>AKEMQNVPYTIAVDGIMAFNQSYLNLPKDSQLSYLDLGNKVKALLYDERGVTPEKIRNAKSAVYTITWKD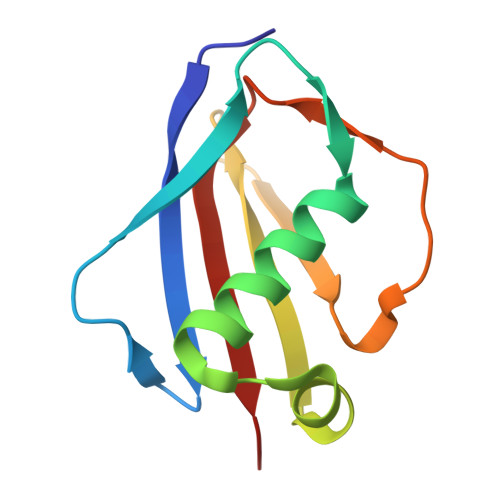GSKKEVDLKKDSYTANLFDSNSIKQIDINVKTK[2x]PYRIDOXAL-5'-PHOSPHATE-N-OXIDE 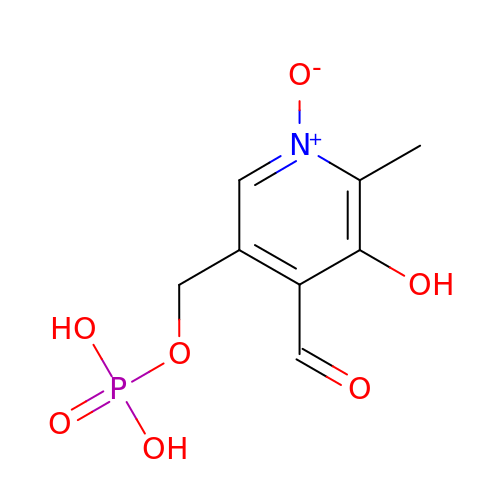| C8 H10 N O7 P | BBWRYPTUKZTWFD-UHFFFAOYSA-N>[2x]GSDELYRQSLEIISRYLREQATGAKDTKPMGRSGATSRKALETLRRVGDGVQRNHETAFQGM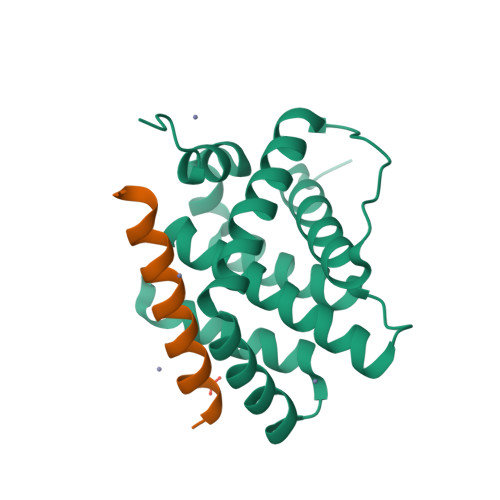LRKLDIKNEDDVKSLSRVMIHVFSDGVTNWGRIVTLISFGAFVAKHLKTINQESCIEPLAESITDVLVRTKRDWLVKQRGWDGFVEFFHVEDLE;>[2x]XQWVREIAAGLRRAADDVNAQVERX> AARMSEQSICQARAAVMVYDDANKKWVPAGGSTGFSRVHIYHHTGNNTFRVVGRKIQDHQVVINCAIPKGLKYNQATQTFHQ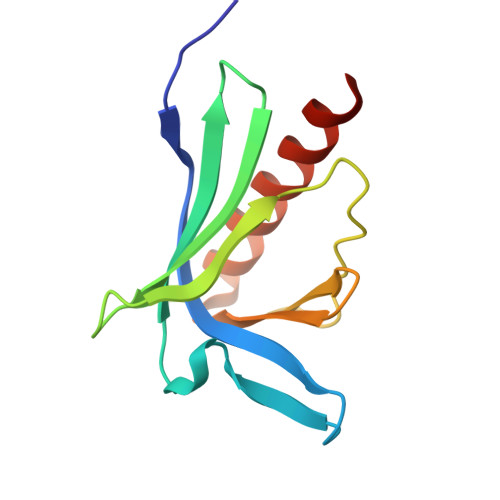WRDARQVYGLNFGSKEDANVFASAMMHALEVLNSQET> SNAMKLKKSPLLLLIITFIFV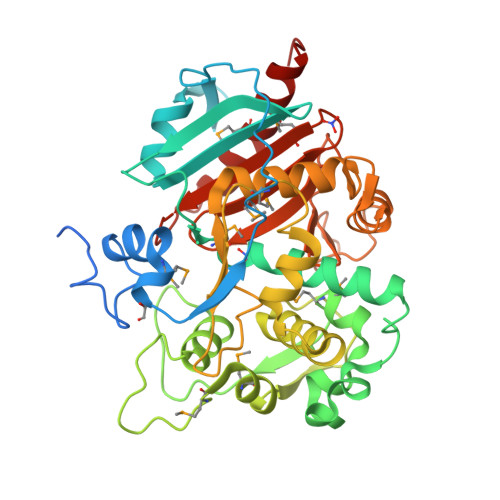ITGLGFTYFKHNKTTPSKNNVTKKNWLDDPYLRWSYTHMKEFTLINDVKNNPDQIARFPSALQNLDDFAVQRRFGSATPLKELLDDNKTDAFVVVHNGQLVYERYFNGYNESEPHGMASLAKVFTGAIIQSLAEENRIDLEKTADTYIKELKNTPFGKATLQQLMDMQVSVEYPTHGYEHPALENQDAQLYLASNILPRDKNYDGPMKIYDMLQEAKETAPPGSVFSYNNGSTETLAWIIRTITGKSLAENVSERIWSQIGMEENAYYVTDETKIEQASAGLNATARDMARFGQLLLNNGEYNGKQILPSSITEDIKNVQEGELAIGPGASISYHNQWWIPHNEQGAFEVLGSYGQTLYIDPKAKMVIVHFSSNATPSNEIHSVYSNMYIDIAHHLEKLPQ>[7x]MNLIPTVIETTNRGERAYD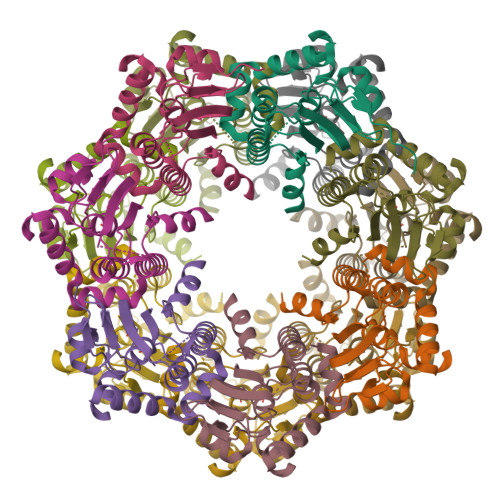IYSRLLKDRIIMLGSQIDDNVANSIVSQLLFLQAQDSEKDIYLYINSPGGSVTAGFAIYDTIQHIKPDVQTICIGMAASMGSFLLAAGAKGKRFALPNAEVMIHQPLGGAQGQATEIEIAANHILKTREKLNRILSERTGQSIEKIQKDTDRDNFLTAEEAKEYGLIDEVMVPETK> SNAMTQFEGFTNLYQVSKTLRFELIPQGKTLKHIQEQGFIEEDKARNDHYKELKPIIDRIYKTYADQCLQLVQLDWENLSAAIDSYRKEKTEETRNALIEEQATYRNAIHDYFIGRTDNLTDAINKRHAEIYKGLFKAELFNGKVLKQLGTVTTTEHENALLRSFDKFTTYFSGFYENRKNVFSAEDISTAIPHRIVQDNFPKFKENCHIFTRLITAVPSLREHFENVKKAIGIFVSTSIEEVFSFPFYNQLLTQTQIDLYNQLLGGISREAGTEKIKGLNEVLNLAIQKNDETAHIIASLPHRFIPLFKQILSDRNTLSFILEEFKSDEEVIQSFCKYKTLLRNENVLETAEALFNELNSIDLTHIFISHKKLETISSALCDHWDTLRNALYERRISELTGKITKSAKEKVQRSLKHEDINLQEIISAAGKELSEAFKQKTSEILSHAHAALDQPLPTTLKKQEEKEILKSQLDSLLGLYHLLDWFAVDESNEVDPEFSARLTGIKLEMEPSLSFYNKARNYATKKPYSVEKFKLNFQMPTLASGWDVNKEKCNGAILFVKNGLYYLGIMPKQKGRYKALSFEPTEKTSEGFDKMYYDYFPDAAKMIPKCSTQLKAVTAHFQTHTTPILLSNNFIEPLEITKEIYDLNNPEKEPKKFQTAYAKKTGDQKGYREALCKWIDFTRDFLSKYTKTTSIDLSSLRPSSQYKDLGEYYAELNPLLYHISFQRIAEKEIMDAVETGKLYLFQIYNKDFAKGHHGKPNLHTLYWTGLFSPENLAKTSI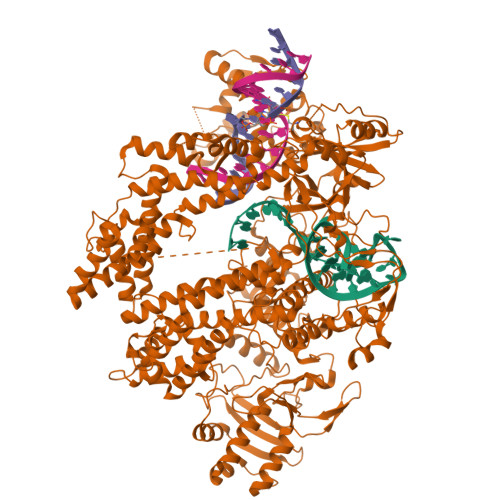KLNGQAELFYRPKSRMKRMAHRLGEKMLNKKLKDQKTPIPDTLYQELYDYVNHRLSHDLSDEARALLPNVITKEVSHEIIKDRRFTSDKFFFHVPITLNYQAANSPSKFNQRVNAYLKEHPETPIIGIDRGERNLIYITVIDSTGKILEQRSLNTIQQFDYQKKLDNREKERVAARQAWSVVGTIKDLKQGYLSQVIHEIVDLMIHYQAVVVLENLNFGFKSKRTGIAEKAVYQQFEKMLIDKLNCLVLKDYPAEKVGGVLNPYQLTDQFTSFAKMGTQSGFLFYVPAPYTSKIDPLTGFVDPFVWKTIKNHESRKHFLEGFDFLHYDVKTGDFILHFKMNRNLSFQRGLPGFMPAWDIVFEKNETQFDAKGTPFIAGKRIVPVIENHRFTGRYRDLYPANELIALLEEKGIVFRDGSNILPKLLENDDSHAIDTMVALIRSVLQMRNSNAATGEDYINSPVRDLNGVCFDSRFQNPEWPMDADANGAYHIALKGQLLLNHLKESKDLKLQNGISNQDWLAYIQELRN> GSDEKRLHFGNGHLKLPGLRTFVDPHTFEDPTQTVHEFAKELDATNISIDKVVGAGEFGEVCSGRLKLPSKKEISVAIKTLKVGYTEKQRRDFLGEASIMGQFDHPNIIRLEGVVTKSKPVMIVTEYMENGSLDSFLRKHDAQFTVIQLVGMLRGIASGMKYLSDMGYVHRDLAARNILINSNLVCKVSDFGLARVLEDDPEAAYTTRGGKIPIRWTSPEAIAYRKFTSASDVWSYGIVLWEVMSYGERPYWEMSNQDVIKAVDEGYRLPPPMDCPAALYQLMLDCWQKDRNNRPKFEQIVSILDKLIRNPGSLKIITSAAARPSN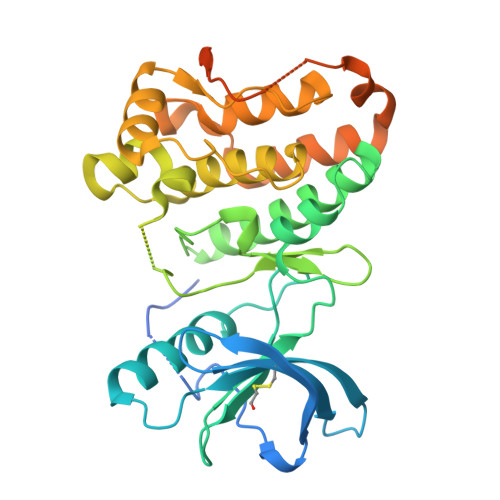LLLDQSNVDITTFRTTGDWLNGVWTAHCKEIFTGVEYSSCDTIAKIS Our study reports on a new class of ferritin-like proteins (EncFtn), which are associated with bacterial encapsulin nanocompartments (Enc). By studying the EncFtn from R. rubrum we demonstrate that iron binding results in assembly of EncFtn decamers, which display a unique annular architecture. Biochemical assays show that EncFtn is active as a ferroxidase enzyme. While EncFtn does not store iron itself, its association with the encapsulin nanocage suggests that mineralization occurs within the cavity of the encapsulin shell (McHugh et al., 2014).

Through site-directed mutagenesis we show that the conserved glutamic acid and histidine residues in the FOC influence protein assembly and activity. Analysis of each of the single mutations (E32A, E62A and H65A) made in the FOC highlights the importance of the iron-coordinating residues in the catalytic activity of EncFtn.

>MAQSSNSTHEPLEVLKEETVNRHRAIVSVMEELEAVDWYDQRVDASTDPELTAILAHNRDEAKEHAAMTLEWLRRNDAKWAEHLRTYLFTEGPITAANSSSVDKLAAALEHHHHHH[30x]> MSAEVIDRFFKSSGAGDIETAVECFADDGQWITPDGDGLGTVHTKDQIG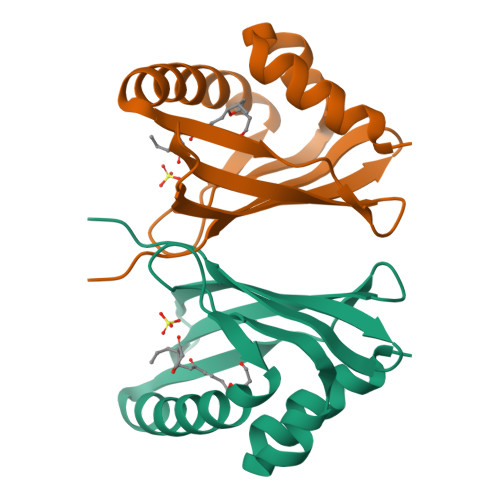DLITSMNAMREKMIASGVDGKFESPIMFGENMGLVRWTVETDDGKVVNRGVDLFILSDGKIVLKDVYRKVKLAAALEHHHHHH> MKTEWPELVGKSVEEAKKVILQDKPAAQIIVL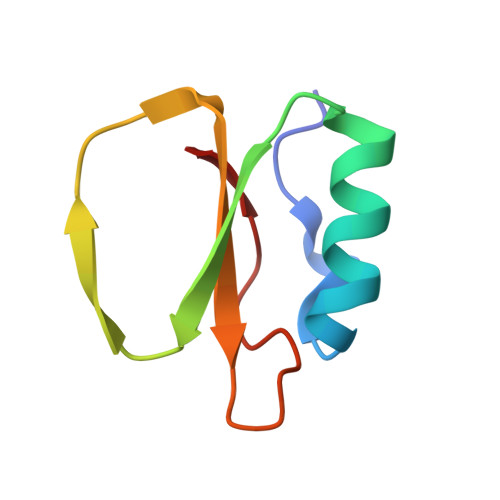PVGTIVTMEYRIDRVRLAVDRLDNIAQVPRVG>MKYLLPTAAAGLLLLAAQPAMAGSDYKDDDDKSGHHHHHHHHHHGSDEVDAGSQQAGTVQDISVVGTTDLLSEFLKTTLTVQPGAALSSVNLRQVEQEVLASGYFKTATAELRTTGGRDTLVVTVTANPVIKDVQATGLTFLPADAFKQSVAELLNIAPGAVLNTQRLEQAKEALAQNYRQEGFPFVPSISADTKTNKDGTATVTFVVDESAPLSRIEVTGATLLPQATVQNIFRPLQTSKRFTTQAFFAASDALQAAYEAAGYFQAGIDPRSVTLENGVLKLSVIESRVASVDLSPLGTLAQTPALQTKAGQPLRLAQLQADVRALANQTGQPVGFALQADPQNPSQVTVLFGAADVESGPVKSIAFVGNTKVPTAQLQAAIKTKPGDVYSPQLAQDDFMALRNVYRQAGYEISTRDAITFQNGVLTYNLREVRLAGYELAWQGQHRTKDRVILRELPAAGQTFNSKDVQAALGRVSALGYVTINDVRVKSDPQNPENVTYVIALSEGRTGIPVNLSLGYDSLQGGWSGDVAYTNSNAFGLGHSFGVRLG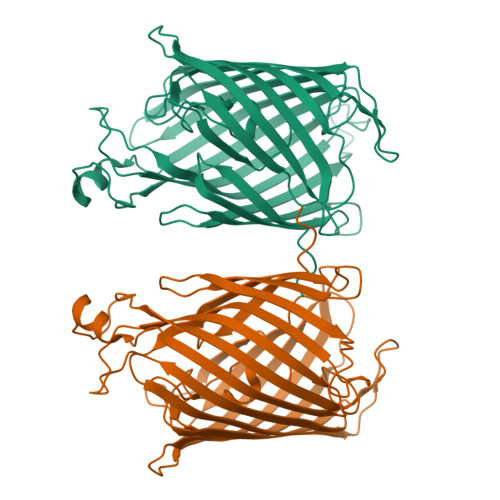AVQNQAGQNWVGSLNYTIPWLDLDFADFRKNRTSLSFGVGSDVGGNIALLDANKEDTGRDYTTRTNGFSLGLGRNITPNLTASANVAFNNRTSYLEPKQEGETSNLDDAAATALLPATSLTTRLSGNLNYDNTDNVNFPGRGVRAYGALGYNVGRAGDAPLSWTDGEIGVSGYYGFGGRIKRSFGLETYRQVLAARANTGTTTGTFPDGTGYFIGGSNPLASRELRGLEDGQLFGTNYFSSSLEYRYDFGLSGGVAQGLYGVLFADYGGVWNSGEAFRSAYGVGAGVQLNLGFGGAQLPSLRFDYGYSGQNAQKPNGRFHFRIGNFW[2x]> MDNLTKVREYLKSYSRLDQAVGEIDEIEAQRAEKSNYELFQEDGVEEHTKPSYFQAADDSDTESEPEIEDNQGLYAQDPEAEQVEGFIQGPLDDYADEEVDVVFTSDWKPPELESDEHGKTLRLTSPEGLSGEQKSQWLSTIKAVVQSAKYWNLAECTFEASGEGVIMKERQITPDVYKVTPVMNTHPSQSEAVSDVWSLSKTSMTFQPKKASLQPLTISLDELFS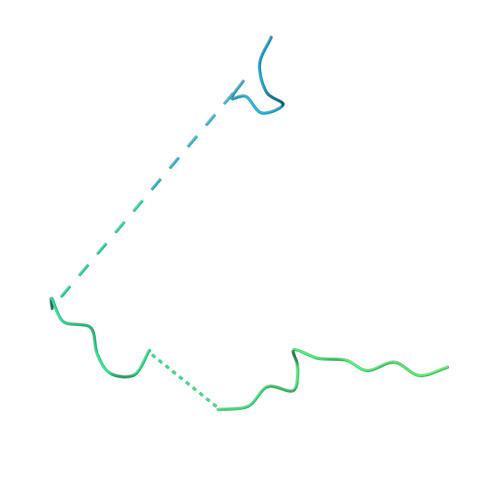SRGEFISVGGDGRMSHKEAILLGLRYKKLYNQARVKYSL>[4x]MKKELYEFYFMPPLKQIEFLEELVNNPEKFKEFFKRLKEEPGAMELFLRNLYLMHPMVQIYFLELLVENPELFKLFFEYLEECPGAMEQFLLNLYLLHPMVQIEFLKLLV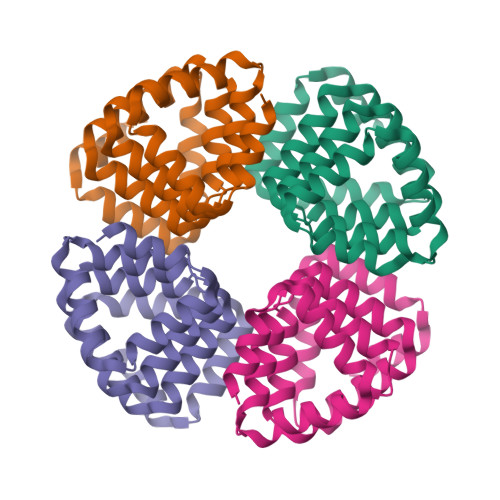ENPELFRLFFEYLKRCPGALELFKEIIELLDPIIQKYLKKLLEENPELKALVKEV> MAEPGIDKLF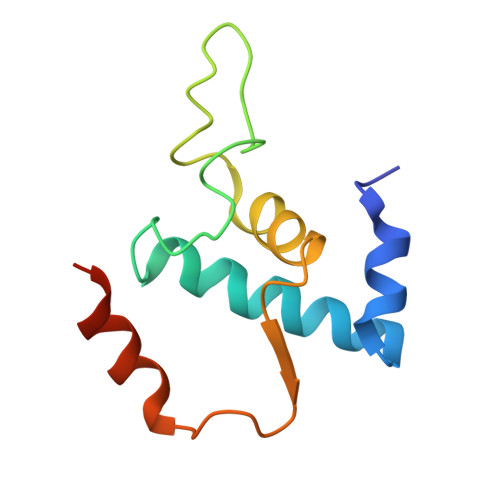GMVDSKYRLTVVVAKRAQQLLRHGFKNTVLEPEERPKMQTLEGLFDDPNAVTWAMKELLTGRLVFGENLVPEDRLQKEMERLYPVEREE6-nitro-L-norleucine | C6 H12 N2 O4 | 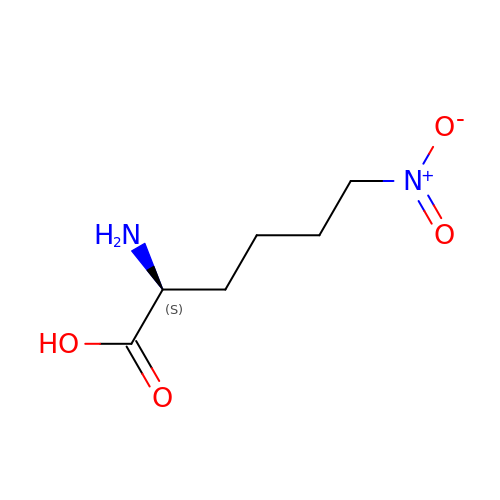LMSAJWJHQUHKSX-YFKPBYRVSA-N> MGSSHHHHHHSAKETFYITTPIYYPSGNLHIGHAYSTVAGDVIARYKRMQGYDVRYLTGTDEHGQKIQEKAQKAGKTEIEYLDEMIAGIKQLWAKLEISNDDFIRTTEERHKHVVEQVFERLLKQGDIYLGEYEGWYSVPDETYYTESQLVDPQYENGKIIGGKSPDSGHEVELVKEESYFFNISKYTDRLLEFYDQNPDFIQPPSRKNEMINNFIKPGLADLAVSRTSFNWGVHVPSNPKHVVYVWIDALVNYISALGYLSDDESLFNKYWPADIHLMAKEIVRFHSIIWPILLMALDLPLPKKVFAHGWILMKDGKMSKSKGNVVDPNILIDRYGLDATRYYLMRELPFGSDGVFTPEAFVERTNFDLANDLGNLVNRTISMVNKYFDGELPAYQGPLHELDEEMEAMALETVKSYTESMESLQFSVALSTVWKFISRTNKYIDETTPWVLAKDDSQKDMLGNVMAHLVENIRYAAVLL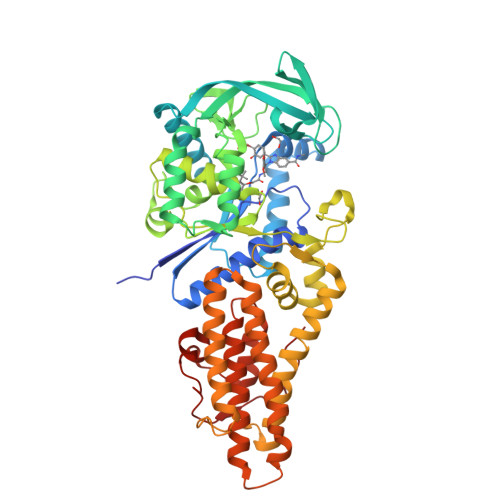RPFLTHAPKEIFEQLNINNPQFMEFSSLEQYGVLNESIMVTGQPKPIFP> MLRKFHVVGISTRIVVNTFGDHNPNGRIYVLKENESKLKDLVRKNPYKPIDLVQPLAIRANEGDIVEILFENQLSFSAGMHFQEADYSVLSSDGADAGYNPDTTVEPGGEILYRLNVNQEGICFFTDLGNVSSTEQGSSVQGLFGALLVQKRGSSWTDPVTGGPINSGVYADIHHPFLPSFREYAWFFNDEMEIRDLTGERPLNPMTNQEAESFHGVNLRYEPMTNRKRLMEAGVVCPDCDSEEVHHDSWVFGDPATPILRGYVGDPAVIRLIHGGVKETHVFHYHVHQWLGDSSNINAEILDAQSISPQTHYSIQPLYGLGSLHGAIGDSIIHCHLYPAFGIGMWGMNRVFDTLQDGSQCYPNGVRIKALMPLPDRPEPPKPTPEKPGFPNFIPGKVGYKAPRPPLGIVGGREMTELERNAAIENPRPGAVFVDPCLDQDPVVVEFNVSAIEMPVVYNKQGWHDPKARFYVMDEDLDDILSGKKEPEPLVFHVPAGTCIRMNYTNRMPHILDGDAFQLVTRTYENGFHIHFVKFDVLACDGGNVGWNYDSAVLPGQTIRYEWYAETELKAFFFHDHLFANSHQQHGVFGAGVIQPRFSKFLDSRTGDEVDHGTQISVEHPLIPDYRDQTLFVHDFALLFDKNGRPIQPPEYPGSEDDPGVFGVNFKCEPLKFRLGEDCDPAYSFSSYVHGDPVTPILRAYEGDPIRIRLLQGAHEESHSFNIHGLRWKEERPDLGSSMKAQQHIGISESFTFETEIPASGDYLWAFEDEEDVWLGTWGLIRAYKGRMEDLIVLTDREALPEGSAETPKPTGKPPEKANPLASLPPGAYQGSPVKKFEVVAFQTPIQYNSYGDHDPYGIIFALKEDVEDILTGKKNPVPLILRANVGDLVEVTLTSELKKELFPFQDGIHPYPPVKEQSFYPPSLRISLHTSLLNYDVKTS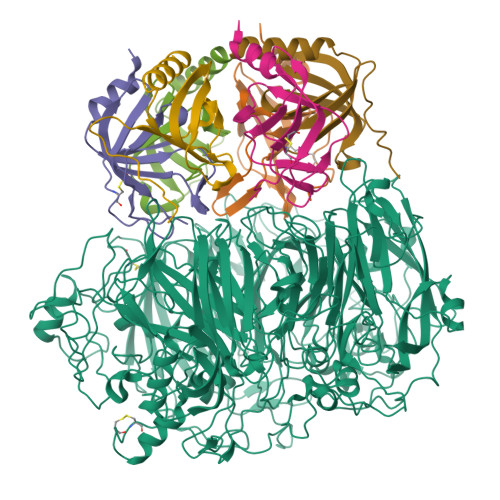SGDTVGYNPDQTVGPGETITYRWFVDGQFGMCSMWDMADLRNHRSFGTFGAFVAESRFTTYLDPYSLEKAITGENVILRHPLLPATREFVLILHDGVRLEDKDGKVIIDPMDGVVPDTEELEEVDTYDYGSRGFNYRSERLINRYKEHPVMHELFSSEVFGDPATPLFEAYPGEPVVMRITTPAERRRAHTFHLHGHYWKFDSKDLDSRIQSFLGHMVTGHTDDLRLIGGAGGVFNFPGDYLYRSGNIRWDIELGMWGIFRVHKDSKENLPRLEEVEGGWDNEEKA;>[3x]MHDSPLKSLSAASNVASVNDPLFDFFNKHMGKQILIITESSQLNILGQTFRPIFCGKVAEVEPGHLTLSPVTIKILNAPFHKFPIPLSIPFEKIAHFTTDVDCSMRIPLV;>[3x]MEALFPMSTDYSKMTDVNEIHDSAILEHFRNGIGHKTLVISPSYPYMFVGIIKELIGDTVMIDVETTHFAQLENREWYIHIHNIEVFYIERPGAPKIPKLEDY>MEIRKDPFTGEYILVSPHRLKRPWQPEGACPFCPGAPETGRGWDVLILPNRYPVVTENPPEPTAEDLYEVIPARGSSLVVVETPQHDVDDLSDLPLGQIKKILTAVAEAQRKAEKEGNAAYFLFFRNKGKEIGVSLTHPFSQIYILPVVPPRVRAELQASYEWYVKHGSCLHCRIVEKEEKRLVFQNRNWKAFVPFYAKWPHEVHIYPKRHRSLLTELTDEEVADLAEALKITLCALKQVAGIPMPYIMVLHQAPLPRPTQYYHLHFE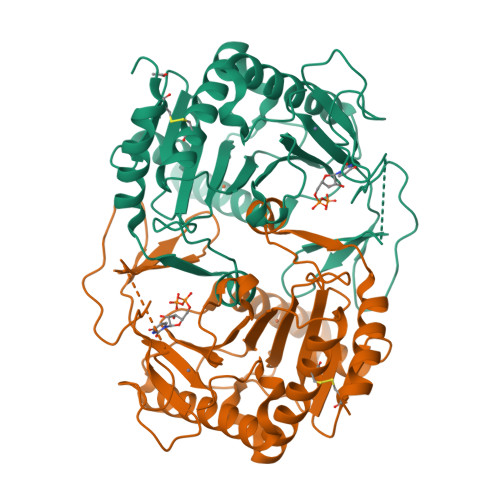IYGMYRPDGKLKHAAGAELGASLFTLDTTPEETAARIKAALQKCLKHSAD[2x]2-[(4-{5-[(4aR,8aS)-3-cycloheptyl-4-oxo-3,4,4a,5,8,8a-hexahydrophthalazin-1-yl]-2-methoxyphenyl}phenyl)formamido]-N-(2-hydroxyethyl)acetamide | C33 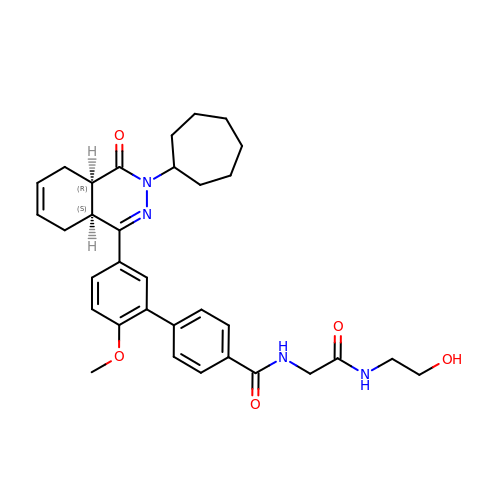H40 N4 O5 | JLYZYBSDRODYRP-RRPNLBNLSA-N>MKVISFLNPKGGSGKTTAVINIATALSRSGYNIAVVDTDPQMSLTNWSKAGKAAFDVFTAASEKDVYGIRKDLADYDFAIVDGAGSLSVITSAAVMVSDLVIIPVTPSPLDFSAAGSVVTVLEAQAYSRKVEARFLITRKIEMATMLNVLKESIKDTGVKAFRTAITQRQVYVKSILDGDSVFESSDGAAKGEIEILTKEIVRIFEATHHHHHH[4x];>[4x]KAHTSVKKMTFGENR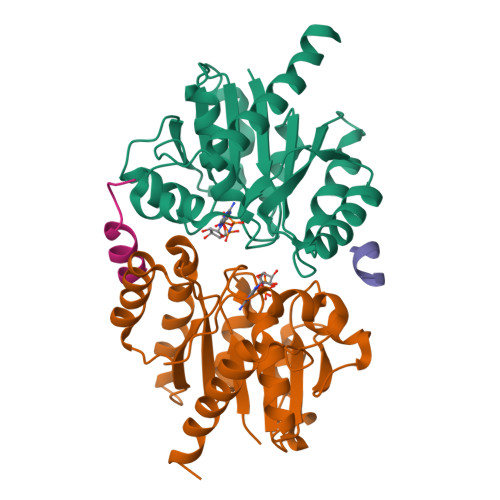DLER> MSGNMDEAVSGNMDEAVSAGKDVRIARWVATIAGLLGFVLSVSIPLLPVTQTTATLNWPQQGRLDNVTAPLISQAPLELTATVPCSVVRDLPPEGGLVFGTAPAEGRDAALNAMLVNVTETRVDVIVRNVVVASVNRDRVAGPDCQRIEITSNLDGTYADFVGLTQISGEDAGKLQRTGYPDPNLRPAIVGVFTDLTGPAPQGLSVSAEIDTRFTTHPTALKLAAMLLAIVSTVIALLALWRLDRLDGRRMHRLIPTRWRTVTAVDGVVVGGMAIWYVIGANSSDDGYILQMARTAEHAGYMANYFRWFGSPEDPFGWYYNVLALMTKVSDASIWIRLPDLICALICWLLLSREVLPRLGPAVAGSRAAMWAAGLVLLGAWMPFNNGLRPEGQIATGALITYVLIERAVTSGRLTPAALAITTAAFTLGIQPTGLIAVAALLAGGRPILRIVMRRRRLVGTWPLIAPLLAAGTVILAVVFADQTIATVLEATRIRTAIGPSQEWWTENLRYYYLIL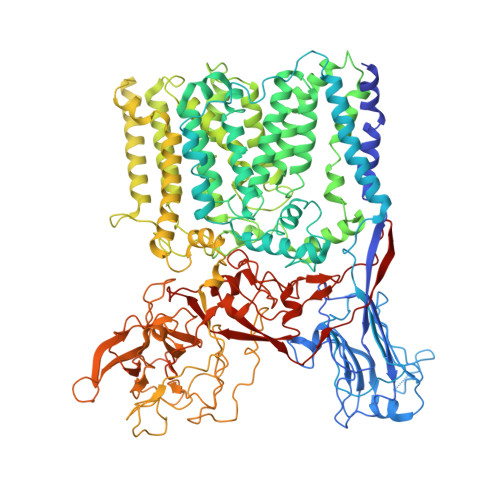PTTDGAISRRVAFVFTAMCLFPSLFMMLRRKHIAGVARGPAWRLMGIIFATMFFLMFTPTKWIHHFGLFAAVGGAMAALATVLVSPTVLRSARNRMAFLSLVLFVLAFCFASTNGWWYVSNFGAPFNNSVPKVGGVQISAIFFALSAIAALWAFWLHLTRRTESRVVDRLTAAPIPVAAGFMVVVMMASMAIGVVRQYPTYSNGWANIRAFAGGCGLADDVLVEPDSNAGFLTPLPGAYGPLGPLGGEDPQGFSPDGVPDRIIAEAIRLNNPQPGTDYDWNRPIKLDEPGINGSTVPLPYGLDPKRVPVAGTYSTEAQQESRLSSAWYELPARDETERAAHPLVVITAAGTITGESVANGLTTGQTVDLEYATRGPDGTLVPAGRVTPYDVGPTPSWRNLRYPRSEIPDDAVAVRVVAEDLSLSQGDWIAVTPPRVPELQSVQEYVGSDQPVLMDWAVGLAFPCQQPMLHANGVTEVPKFRISPDYYAKLQSTDTWQDGINGGLLGITDLLLRASVMSTYLSQDWGQDWGSLRKFDTVVEATPAELDFGSQTHSGLYSPGPLRIRP> SEFLVDRSKNGLIHVPKDLSQKTTILNISQNYISELWTSDILSLSKLRILIISHNRIQYLDISVFKFNQELEYLDLSHNKLVKISCHPTVNLKHLDLSFNAFDALPICKEFGNMSQLKFLGLSTTHLEKSSVLPIAHLNISKVLLVLGETYGEKEDPEGLQDFNTESLHIVFPTNKEFHFILDVSVKTVANLELSNIKCVLEDNKCSYFLSILAKLQTNPKLSNLTLNNIETTWNSFIRILQLVWHTTVWYFSISNVKLQGQLDFRDFDYSGTSLKALSIHQVVSDVFGFPQSYIYEIFSNMNIKNFTVSGTRMVHMLCPSKISPFLHLDFSNNLLTDTVFENCGHLTELETLILQMNQLKELSKIAEMTTQMKSLQQLDISQNSVSYDEKKGDCSWTKSLLSLNMSSNILTDTIFRCLPPRIKVLDLHSNKIKSIPKQVVKLEALQELNVASNQLKSVPDGIFDRLTSLQKIWLHTNPWDCSCPRIDYLSRWLNKNSQKEQGSAKCSG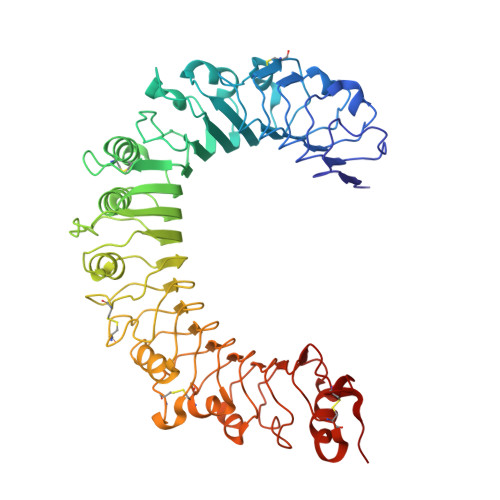SGKPVRSIICP> TPAFNKPKVELHVHLDGAIKPETILYFGKKRGIALPADTVEELRNIIGMDKPLSLPGFLAKFDYYMPVIAGCREAIKRIAYEFVEMKAKEGVVYVEVRYSPHLLANSKVDPMPWNQTEGDVTPDDVVDLVNQGLQEGEQAFGIKVRSILCCMRHQPSWSLEVLELCKKYNQKTVVAMDLAGDETIEGSSLFPGHVEAYEGAVKNGIHRTVHAGEVGSPEVVREAVDILKTERVGHGYHTIEDEALYNRLLKENMHFEVCPWSSYLTGAWDPKTTHAVVRFKNDKANYSLNTDDPLI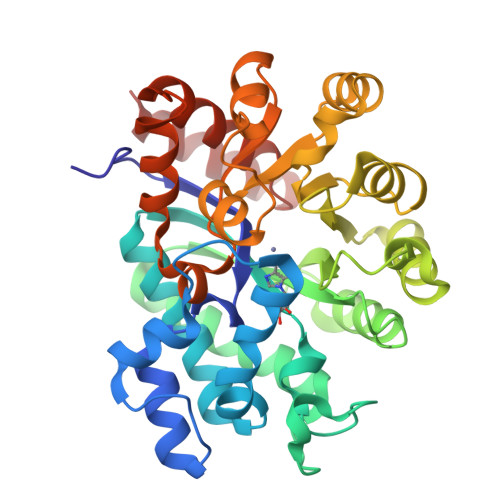FKSTLDTDYQMTKKDMGFTEEEFKRLNINAAKSSFLPEEEKKELLERLYREYQ> P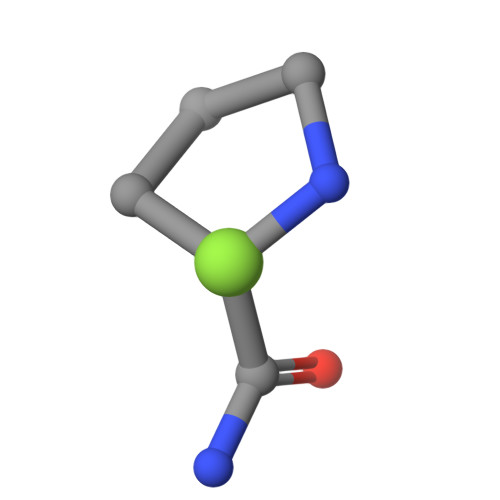GG> MQLETAELEKGIVRVLVDVIGHRLARDKNN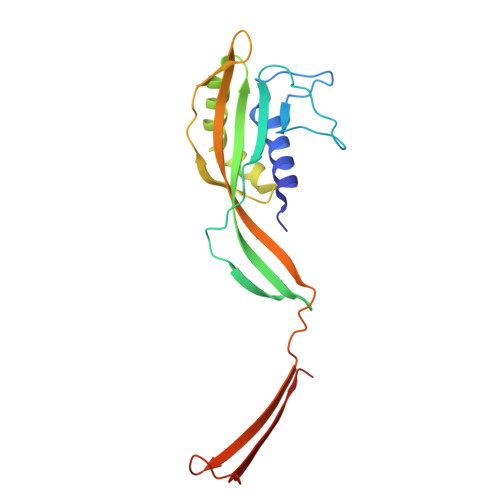RPNVIRAYPSDNSNDKGLKPDQPFITVYCQDATTPYGWVLDKFVEDDAVCYRIAFQIPVLITVNGKGAHSIMLELKQRLEMSTTRDYLADMTGASVLDTGAIPNDYTYLNTDFENSAPLVVTLVKNSVLKDERGSIIERVIVDGELVYEEGQEPPEYTIHLDVDSKGVK>[4x]GIGTGFPFDPHYVEVLGERMHYVDVGPRDGTPVLFLHGNPTSSYVWRNIIPHVAPTHRCIAPDLIGMGKSDKPDLGYFFDDHVRFMDAFIEALGLEEVVLVIHDWGSALGFHWAKRNPERV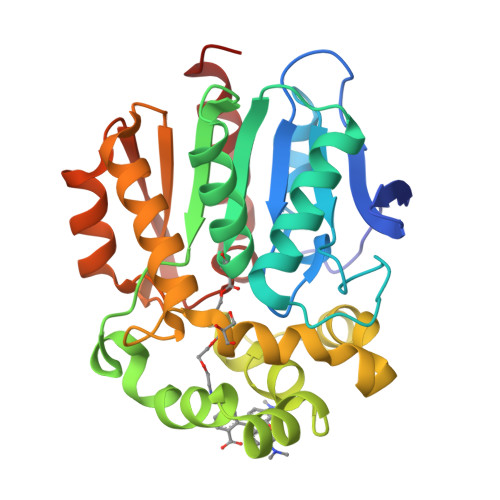KGIAFMEFIRPIPTWDEWPEFARETFQAFRTTDVGRKLIIDQNVFIEGTLWMGVVRPLTEVEMDHYREPFLNPVDREPLWRFPNELPIAGEPANIVALVEEYMDWLHQSPVPKLLFWGTPGVLIPPAEAARLAKSLPNCKAVDIGPGLNLLQEDNPDLIGSEIARWLSTLEI>MAPQEQASSSQQDDAPPKTPNVVEPYKGEVAICGLSGRYPESANVGELEYNLFNKIDMVTIDNRRWEPGYLGTPERMGKVKTITDFDAEFFGVHTKGAQTMDPMLRNLLEVVYEAIVDAGESLESMKGTRTGVYIGVSNNEVDTAYMKNWTDDDAYMVQGCHHSMYPNWISFFFDFSGPSTAYNTACSTSLVCLDAAERHLRMGVIDNAIVGGSNFIYRPATTKLFMGMNFLGSSTCKAFDESGDGFVRGEVASAILLKKADTAKRVYCTLVGSMLNNDGNQTNGILYPNSEAQEQLMTDIYSTHKIDANEVKYFECHGTGTQAGDPNETRAICNAVCKGKKDPLLIGSIKSNLGHGETASGINGISKVIITMHSRQIPPNLHFKNPNPKIPGLFDGRLKVVTETTPFDGGLIAINSFGMGGTNAHAIFRSFDKRAEPHPASDKPRLFTYCARTEEGLQKIFEEAHKHASNVEFHALCQESANTKPKSLPYRGATILNAEGEYTEIQKCPSKAREVWFVYSGMGSQWVGMGRSLMALDVFRQSIEETAAILSPFGVDLMSLLMDGTEDKLKEIMPPFICINAIQLALTDLLNS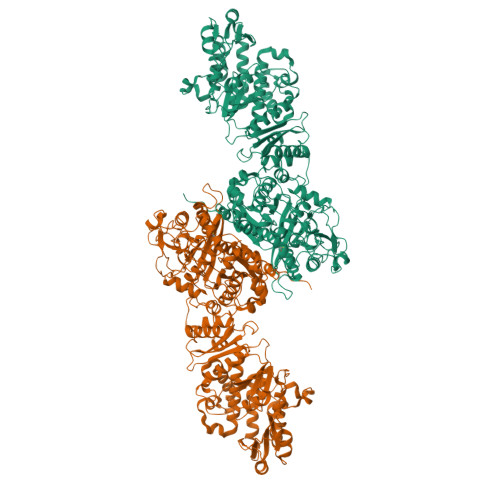MGIVPDGLVGHSLGEVGCAYADGCLTRREAILSAFWRAKAVIDCEVKPGKMAAVELTWEEAKRLCPPGVVAACHNSQDSVTISGGAQEMTKFMAELSAQGVTVKEVNSNNISYHSSFMTEPAAYLKKGLEKEIVPKPRSKKWISTSIPEERWGNPEAQTADASYQANNLLSSVLFYEGLQKIPSNAIAIEIAPAGLLQSVIKKSLGQDCTIVALQKRKSPNNLEVFFSALGKCYSHGVPMNPLGLYPAVQFPVSIDTPMLSSMVSEAWDHSAKWRVPLVEEFEYGSGSSSDNVIDIDLSEDSPENYLLEHAVDGRMLFPATGTLVLAWKTLAKLKGVEFEQLGVQMTNVQIHQALFLNPGGKTTVSVSVMPITGEFQVRDGESLISSGVITSSEGRLLETDQHMKKGSVLDGKPDKELLFTKEIYREFLLRGYEYGAAFQGIQRASLDATDTDIRWDGRWISYLDTVLQMYLLSKPGTHQALPTLLESVTIDPRVHPAQPPEGTTEFQVLPGKWDPVLQIAAAGGVEIRSCHSIRASRRLNHDPPILEDFAFAPYVDPRPSDRSAAAVTPALRDYADACFEFSRQGMKRWLENDKNNVLPNKEEIKEALAMANKHASTPQAASNFASAKATLEALVNNKNGHRLPNHGLFEMLDIAFSEPLEGDYWDRLRMKLHDVRTYLWDDPIIAALESPDIVKLVMETVSDNVNQQVMEILEVGAARGPYYRQAIPKALEYFSIKDWQYTVADQGFVEDAAEFPVKMMQFDPLDPANFPAELTESCDLLVLKWNLQMQVDLDAAITEFSKMIKPGGFLLVLENGTRLSTFFPIKAIVSASLGGKGGPEGDRAMGCFYTDAQWSALFARHGFEQIMHIPDGIAVSMFLLRKPFEPSVAPIIINVDDLECSWLEEVQARCAELQDSHKDSRLWLVANTELSGVLGFLRSLVWEFGSEKLRCIQIDDATAGPNPPKISADSADFKELVRKDLAYNVFKNGKWGTYRGFVISDADRQKERPSEYVYADWLSAGDMSSLRWFDSPLKTGHNNGMLGSKMAHKLETETCSVYYAGLNLRDIILANGTIQRDILPEETFFKEGVLGVEFSGRNSSGKRVMGLCPPPALATTVKCPVSSLWSVPDQWTLEEAATVPLAYATAYYCLVSEGGVQKGATVFIHAGASVVGQASIAVALSYNCEIFTLTKNSDETALLKSMYPQLNDRNFCSSEDCSFEKYIRKETKGSGVDVVINTLRGKFLKASRRLLSKKGKFVDIGFKVDSNTQIAYYTREHPDLRFQLDALLESQGPEWTRLFDLVQAGIHSGVVKPLKRAVYSMDKIVDAFKTVEAEREAGKIVIKIRDEERQKVCPTPRTSFPAIHRTCFHPDKSHILVGGMGGMGLETAHWMVLRGAKKLILTSRYGITTGYQARKIAFFKQLGVEVEVLALSVNTRKAADKVFEHALKMGPVGGIFNMAMVLYNDDFLKMNREQFLKPLESKITMTMLLDDKSREKPVRDTLDHFVMFSSLIVSGGHLGQANYAFGSTVLEKICERRKRDGLPVTTPQWASIADVGTVALMGTGNETIICRKYPQRFFNVLSVFDFMMSSDNVVTISYVLVEKSMGVAAGEESMVDQVLRAVGKVLGIKDVSSVDGDKEFIDMGVDSLMSVEIKQALERDAGLVISTKDTQLMTFNTLRSMVKGSHVHHHHHH[2x]>[4x]AEFSRHSEKIAIRDFQVGDLVL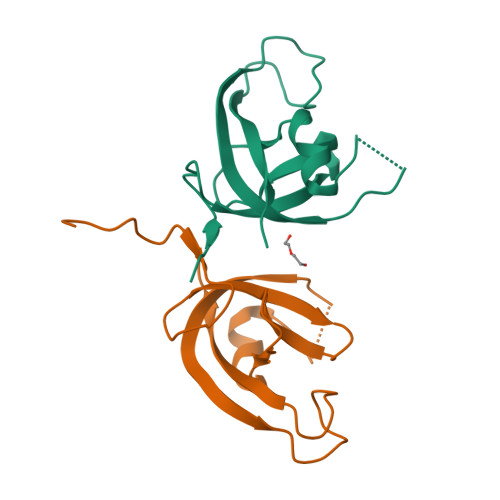IILDERHDNYVLFTVSPTLYFLHSESLPALDLKPGEGASGASRRPWVLGKVMEKEYCQAKKAQNRFKVPLGTKFYRVKAVSWNKKV> MSIDTARSGSDDDVEIREIQAAAAPTRFARGWHCLGLLRDFQDGKPHSIEAFGTKLVVFADSKGQLNVLDAYCRHMGGDLSRGEVKGDSIACPFHDWRWNGKGKCTDIPYARRVPPIAKTRAWTTLERNGQLYVWNDPQGNPP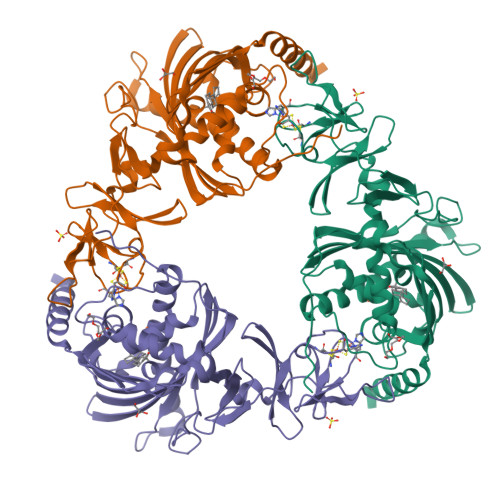PEDVTIPEIAGYGTDEWTDWSWKSLRIKGSHCREIVDNVVDMAHFFYIHYSFPRYFKNVFEGHTATQYMHSTGREDVISGTNYDDPNAELRSEATYFGPSYMIDWLESDANGQTIETILINCHYPVSNNEFVLQYGAIVKKLPGVSDEIAAGMAEQFAEGVQLGFEQDVEIWKNKAPIDNPLLSEEDGPVYQLRRWYQQFYVDVEDITEDMTKRFEFEIDTTRAVASWQKEVAENLAKQAEGSTATP>MLTETEGRAAVKLARKTIEIFLSKGKSPRPDASGVELSPVFEEYRGVFVTLTEGGLLRGCIGHPYPDSTLKEAILDSAISAATRDPRFPTVEQDEMKNILVEVTILTQPEKINASPKELPDKVEIGKHGLIVKQGYCQGLLLPQVAPENDMDSIDFLSHTCMKAGLSPDAWVKGAEVYCFEGQIFKEKEPDGEVIE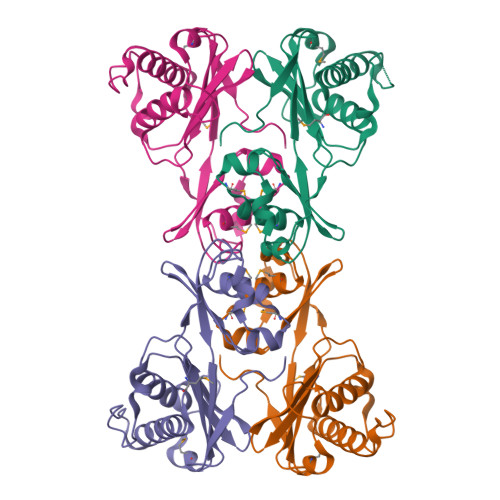EKFLEHHHHHH[4x]(2R,3S,4S,5S)-2,3,4,5-tetrahydroxyhexanoic 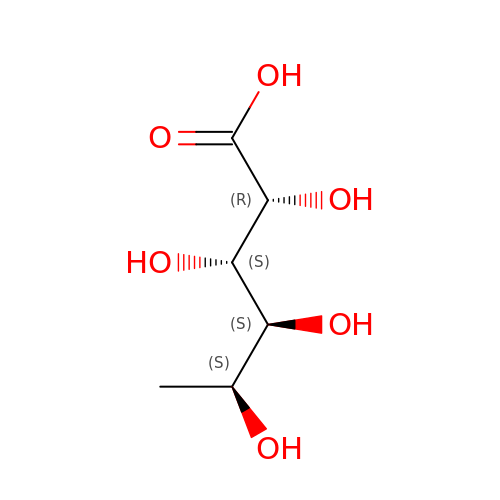acid | C6 H12 O6 | NBFWIISVIFCMDK-NEEWWZBLSA-N> SGISLDNSYKMDYPEMGLCIIINNKNFHKSTGMTSRSGTDVDAANLRETFRNLKYEVRNKNDLTREEIVELMRDVSKEDHSKRSSFVCVLLSHGEEGIIFGTNGPVDLKKITNFFRGDRCRSLTGKPKLFIIQACRGTELDCGIETD;> DMACHKIPVDADFLYAYSTAP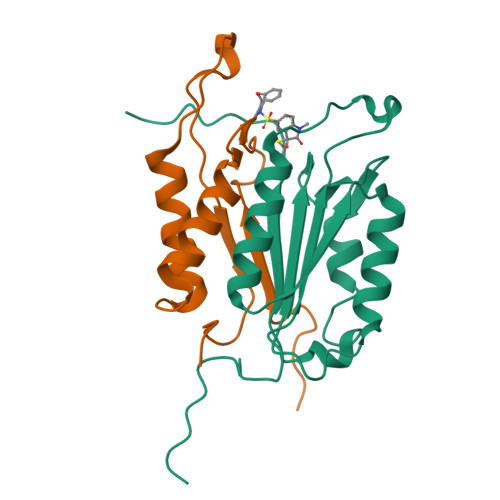GYYSWRNSKDGSWFIQSLCAMLKQYADKLEFMHILTRVNRKVATEFESFSFDATFHAKKQIPCIVSMLTKELYFYH> MKMDKKTIVWFRRDLRIEDNPALAAAAHEGSVFPVFIWCPEEEGQFYPGRASRWWMKQSLAHLSQSLKALGSDLTLIKTHNTISAILDCIRVTGATKVVFNHLYDPVSLVRDHTVKEKLVERGISVQSYNGDLLYEPWEIYCEKGKPFTSFNSYWKKCLDMSIESVMLP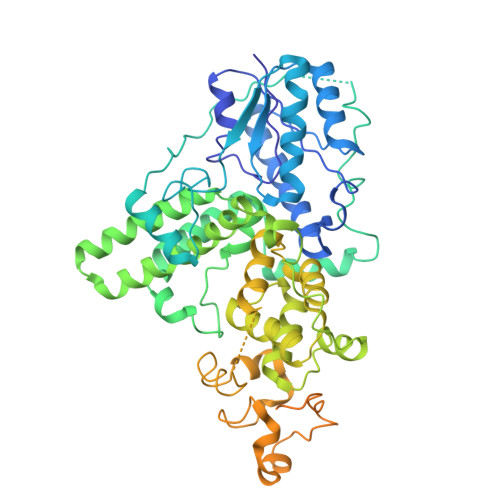PPWRLMPITAAAEAIWACSIEELGLENEAEKPSNALLTRAWSPGWSNADKLLNEFIEKQLIDYAKNSKKVVGNSTSLLSPYLHFGEISVRHVFQCARMKQIIWARDKNSEGEESADLFLRGIGLREYSRYICFNFPFTHEQSLLSHLRFFPWDADVDKFKAWRQGRTGYPLVDAGMRELWATGWMHNRIRVIVSSFAVKFLLLPAKWGMKYFWDTLLDADLECDILGWQYISGSIPDGHELDRLDNPALQGAKYDPEGEYIRQWLPELARLPTEWIHHPWDAPLTVLKASGVELGTNYAKPIVDIDTARELLAKAISRTREAQIMIGAAPDEIVADSFEALGANTIKEPGLCPSVSSNDQQVPSAVRYNGSKRVKPEEEEERDMKKSRGFDERELFSTAESSSSSSVFFVSQSCSLASEGKNLEGIQDSSDQITTSLGKNGCK methyl (2R)-2-(phenylmethoxycarbonylamino)-3-sulfanyl-propanoate | C12 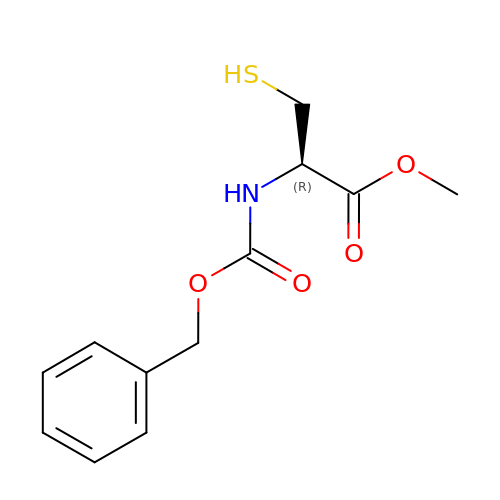H15 N O4 S | FEADQZMKQOMOMD-JTQLQIEISA-N>GPGSMLRAANLDRSPEEYGMGSLDGRVVFITGAARGQGRSHAVMCAEQGANIVGVDICEDIDIVPYKLGTYEELEETARLVEKTGQEMLFRKADVRDKAVLQEVFDAGVEQFGHIDTVIANAGVVLTNPDERDASEALRLGLDIMLIGVWNTFQVAIPHMKERGQGGNLIATSSMIALLDLTDGRGGTDAYLTSKLAITGLVRSYALMLAADRIRVNGVAPTNCSTPMITENPALFKVIEENPHLVNAMSTALPDFPMIEPRDVSNAILFLISDAGRSFTGSVLKVDAGMDVKR[2x]

Here we present a series of TIGR03971 SDR crystal structures from several mycobacterial species which contain an insertion in the primary sequence at the NAD cofactor binding site. These crystal structures demonstrate that the inserted protein residues almost completely cover the NAD cofactor, only leaving part of the nicotinamide ring exposed to solvent. NMR experiments did not show exchange of the NAD cofactor, whereas binding was demonstrated for a number of small molecules which could be potential substrates, products, inhibitors, or artificial redox partners. Experimental results are consistent with the notion that the SDR family enzymes linked by comparative genomics studies to mycofactocin do indeed keep their NAD tightly bound beneath a protein structure that may interact with a specialized adaptor machinery for redox exchange.

With the exception of the M. thermoresistibile target which did not contain NAD, all other mycobacterial SDR target crystal structures contained NAD, which appears to have co-purified with the protein after expression in E. coli. For each of these crystal structures, the adenosine mononucleotide portion of the cofactor binding site is enveloped by the inserted residues and only a portion of the nicotinamide ring appears open to solvent (see representative examples in Fig. 2A and B). In addition to the insertion loop which covers the adenosine portion of the cofactor, a second loop which typically contains two α-helices covers much of nicotinamide mononucleotide portion of the cofactor. In contrast, this loop is ordered in each of the mycobacterial SDR crystal structures presented here. The combination of the insertion loop which covers the adenosine portion of the cofactor and the ordering of the second loop which covers the nicotinamide mononucleotide portion of the cofactor results in a significant decrease in the solvent accessible surface area of the cofactor in the mycobacterial SDRs, relative to other NAD- and NADP-dependent dehydrogenases. Only a small portion of the nicotinamide ring appears available to solvent in each of these cases, indicating that the NAD cofactor is tightly bound and potentially non-exchangeable. The structures presented here have a cofactor solvent accessible surface area of approximately 18 Å2, whereas other NAD- or NADP-bound dehydrogenases have a cofactor solvent accessible surface area of 82–89 Å2. Given the encapsulation of the NAD cofactor by the two loops in mycobacterial SDRs, a large conformational change would be required to release the NADH cofactor after a redox reaction had occurred. To test whether or not the bound NAD was exchangeable, we performed a number of line broadening and STD-NMR ligand-observe studies, and did not observe exchange of NAD/NADH during the timescale of the NMR experiments.>GSHMISEHDSVLEKYPRIQKVLNSTVPALSLNSSTRYEGKIINIGGTIIKARLPKARIGAFYKIEPSQRLAEVIAIDEDEVFLLPFEHVSGMYCGQWLSYQGDEFKIRVGDALLGRLIDGIGRPMESNIVAPYLPFERSLYAEPPDPLLRQVIDQPFILGVRAIDGLLTCGIGQRIGIFAGSGVGKSTLLGMICNGASADIIVLALIGERGREVNEFLALLPQSTLSKCVLVVTTSDRPALERMKAAFTATTIAEYFRDQGKNVLLMMDSVTRYARAARDVGLASGEPDVRGGFPPSVFSSLPKLLERAGPAPKGSITAIYTVLLESDNVNDPIGDEVRSILDGHIVLTRELAEENHFPAIDIGLSASRVMHNVVTSEHLRAAAECKKLIATYKNVELLIRIGEYTMGQDPEADKAIKNRKLIQNFIQQSTKDISSYEKTIESLFKVVA[6x];> GSHMLDRILSIRKSRANRLRESMAKINSQIKEVDGKLDDCEQSIKESIASKQAYCASLVNLDKVSLYKYQ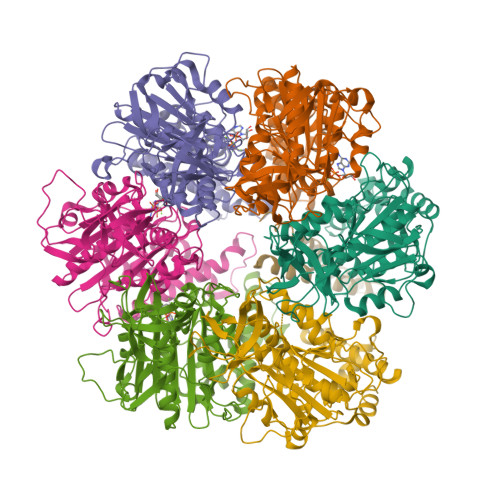IKNNAFDEQKQRLYEKKSSLSKEKRSLLDSQKRTKENLQHVNKSVEKLSFAIKEHYFD>NEDMPVERILEAELAVEPKTETYVEANMGLNPSSPNDPVTNICQAADKQLFTLVEWAKRIPHFSELPLDDQVILLRAGWNELLIASFSHRSIAVKDGILLATGLHVHRNSAHSAGVGAIFDRVLTELVSKMRDMQMDKTELGCLRAIVLFNPDSKGLSNPAEVEALREKVYASLEAYCKHKYPEQPGRFA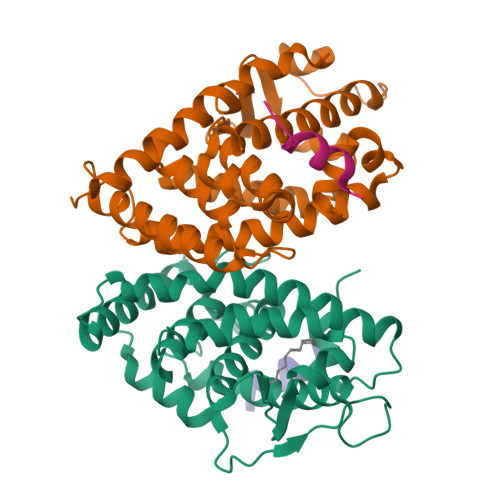KLLLRLPALRSIGLKCLEHLFFFKLIGDTPIDTFLMEMLEAPHQMT[2x];>PVQLSKEQEELIRTLLGAHTRHMGTMFEQFVQFRPPAHLFIHHQPLPTLAPVLPLVTHFADINTFMVLQVIKFTKDLPVFRSLPIEDQISLLKGAAVEICHIVLNTTFCLQTQNFLCGPLRYTIEDGARVGFQVEFLELLFHFHGTLRKLQLQEPEYVLLAAMALFSPDRPGVTQRDEIDQLQEEMALTLQSYIKGQQRRPRDRFLYAKLLGLLAELRSINEAYGYQIQHIQGLSAMMPLLQEICS[2x];>[4x]ERHKILHRLLQEG>RRNMFQGIEDPDRIERAFNLPLYGLVPQSAEQ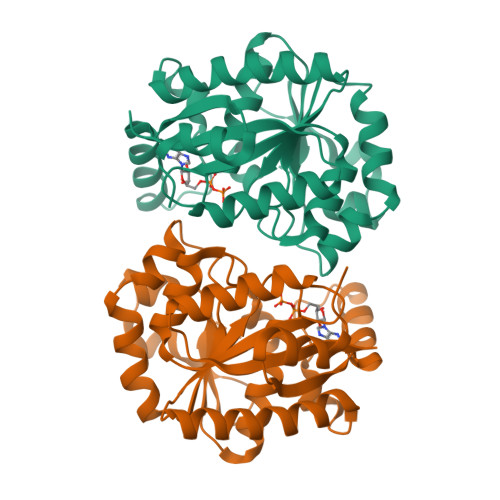VKLDAQAEKSGSRTRPILASLRPKDLSVESLRSLRTAMQFAMMDAKNRVIVLTGPTPGIGKSFLTVNLAVLLAHSGKRVLLIDADMRRGLLDRYFGLTSQPGLSELLSDQSALEDAVRETPVQGLSFISAGTRPPNPSELLMSTRLPQYLEGLGKRYDVVLIDSPPVLAVTDATIIGRMAGSTFLVLRSGMHTEGEIADAIKRLRTAGVDLEGGIFNGVPPKARGYGRGYAAVHEYLSA[2x]> GPLGSPEFMARTLQGEWMKVEQKGGQVPAPRSSHGIAVIGDKLYCFGGEDPPYESIDNDLYVFDFNTHTWSIAPANGDVPKTRVLGTRMVAVGTKLYVFGGRNKQLEFEDFYSYDTVKEEWKFLTKLDEKGGPEARTFHSMTSDENHVYVFGGVSKGGLNATPFRFRTIEAYNIAEGKW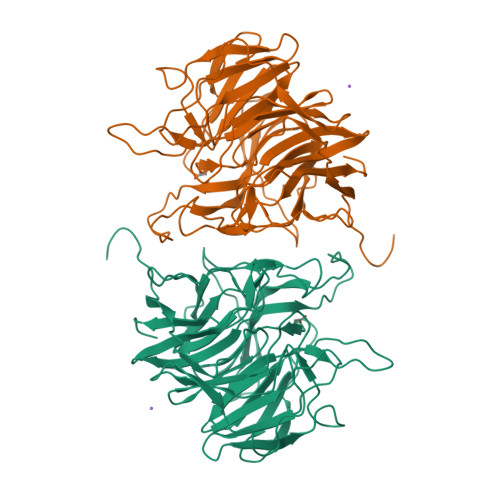AQLPDPGEDFEKRGMAGFLVVQGKLWVFYGFATANDPKIPTLYGSQDYESNRVHCYDPATQKWTEVETTGFEKPSRRSCFAHAAVGKYIIIFGGEIERDPEAHQGPGTLSREGFALDTETLVWERYEGGPIKPSNRGWVASTTTTINGKKGLLVHGGKLMTNERTDEMYFFAVNSST(E)-3-(4-methoxyphenyl)acrylic acid | C10 H10 O3 | 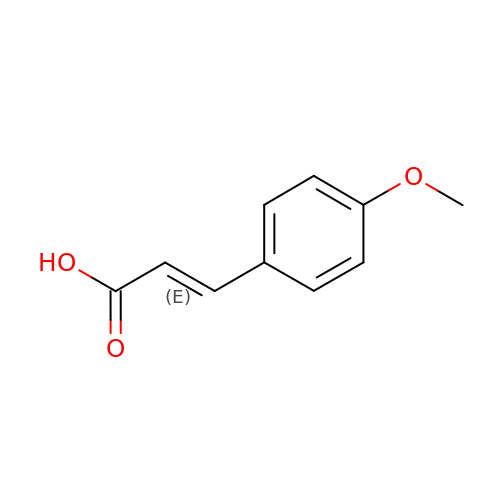AFDXODALSZRGIH-QPJJXVBHSA-N The mammalian family of secreted phospholipase A2 (sPLA2), which are Ca2+ dependent, low-molecular weight and disulfide-rich enzymes, plays key roles in many physiological functions and pathological processes by catalyzing the hydrolysis of phospholipids at the sn-2 position. GIIE, the closest homolog to GIIA, is regarded as a “hair follicular”, “inflammatory” and “metabolic” sPLA2. The structure of hGIIE consists of a typical set of three major helices (α1, α3 and α4), two β-strands (β1 and β2), and three short helices (α2, α5 and α6) around the second calcium binding site. Similar to hGIIA, hGIIE has seven disulfide bonds.

Two are apo-hGIIE structures at the resolution of 2.0 Å and 1.9 Å, with different crystallization conditions: without (apo-hGIIE_1) or with calcium (apo-hGIIE_2). In the hGIIE-LY311727 complex structure, Ca1 is 100% occupied, with the extra two coordination from the amide oxygen and phosphate oxygen in LY311727. In the apo-hGIIE_2 structure, crystallized in the presence with 10 mM CaCl2, Ca1 with 100% occupancy is seven-coordinated, and two water molecules provide the extra two coordination. In the apo-hGIIE_2 structure, Ca2 is 39% occupied and coordinated by carbonyl oxygen of Gly24, Tyr111, three water molecules, and either the carbonyl or carboxyl oxygen of Asp22. Amide oxygen in the 3-side chain and one of the carboxyl oxygen in the 4-side chain of inhibitors are coordinated with calcium instead of water in the apo-hGIIE_2 structure. Similarly in apo-hGIIE structures, a water molecule, part of the second calcium hydration shell, forms a hydrogen bond to the carbonyl oxygen of Cys27 and links the second calcium to the oxyanion.

> NLVQFGVMIEKMTGKSALQYNDYGCYCGIGGSHWPVDQTDWCCHAHDCCYGRLEKLGCEPKLEKYLFSVSERGIFCAGRTTCQRLTCECDKRAALCFRRNLGTYNRKYAHYPNKLCTGPTPPC> GTTVTDCTPGPNQNGVTSVQGDEYRVQTNEWNSSAQQCLTINTATGAWTVSTANFSGGTGGAPATYPSIYKGCHWGNCTTKNVGMPIQISQIGSAVTSWSTTQVSSGAYDVAYDIWTNSTPTTTGQPNGTEIMIWLNSRGGVQPFGSQTATGVTVAGHTWNVWQGQQTSWKIISYVLTPGATSISNLDLKAIFADAAARGSLNTSDYLLDVEAGFEIWQGGQGLGSNSFSVSVTSGASHHHHHH

GuxA is a multi-modular and multi-functional enzyme from Acidothermus cellulolyticus whose catalytic domains include a xylanase/endoglucanase GH12 and an exoglucanase GH6, representing a unique combination of these two glycoside hydrolase families in a single CAZyme. GuxA on the other hand contains an N-terminal GH6 domain linked to a CBM3 followed by a GH12 catalytic domain linked to a CBM2 on the C-terminal end. GuxA shows an optimal temperature range between 75 and 80 °C for all three substrates, which is well above the optimal growth temperature of 55 °C for A. cellulolyticus.

The structure of the GuxA GH12 domain was solved with and without cellobiose bound in the active site, to resolutions of 1.5 and 1.85 Å, respectively. The domain exhibits the classic GH12 β-jelly roll, with two curved β-sheets packed together-their concave face forming the active site-and one α-helix. The active site cavity is lined with aromatic residues that accommodate the substrate without any significant change in structure at the local or whole-protein level—The Cα RMSD between the structures with and without cellobiose bound is 0.166 Å. The reducing end of the bound cellobiose is sandwiched between two loops formed by residues Thr59-Pro63 and Val142-Phe145, and primarily contacts the peptide backbone atoms of these residues. Glu131 and Glu216 are the catalytic residues (the nucleophile and the general acid/base, respectively), whereas the strictly conserved active site aspartate residue is at position 114. In the case of the A. cellulolyticus GuxA GH12 domain, the leucine at this position probably makes a modest contribution to the enzyme’s thermal stability which, along with the extra disulfide bond, accounts for the thermotolerance of the enzyme.> GAKPYEKVRIYRMDGSYRSVELKHGNNTTVQQIMEGMRLSQETQQYFTIWICSENLSLQLKPYHKPLQHVRDWPEILAELTNLDPQRETPQLFLRRDVRLPLEVEKQIEDPLAILILFDEARYNLLKGFYTAPDAKLITLASLLLQIVYGNYESKKHKQGFLNEENLKSIVPVTKLKSKAPHWTNRILHEYKNLSTSEGVSKEMHHLQRMFLQNCWEIPTYGAAFFTGQIFTKASPSNHKVIPVYVGVNIKGLHLLNMETKALLISLKYGCFMWQLGDTDTCFQIHS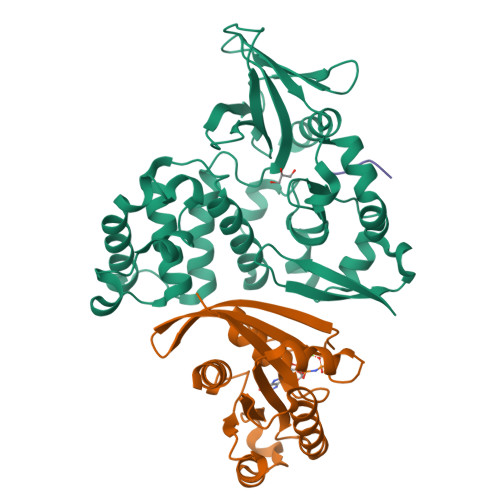MENKMSFIVHTKQAGLVVKLLMKLNGQLMPTERNS;> MREYKLVVLGSGGVGKSALTVQFVQGIFVEKYDPTIEDSYRKQVEVDAQQCMLEILDTAGTEQFTAMRDLYMKNGQGFALVYSITAQSTFNDLQDLREQILRVKDTDDVPMILVGNKCDLEDERVVGKEQGQNLARQWNNCAFLESSAKSKINVNEIFYDLVRQINR;> SRHSCIFPGQYNPSFISDESRRRDYF>[2x]MGLASLADFPIGVAVAASGGNADIFTSSARQNIVRAEFNQITAENIMKMSYMYSGSNFSFTNSDRLVSWAAQN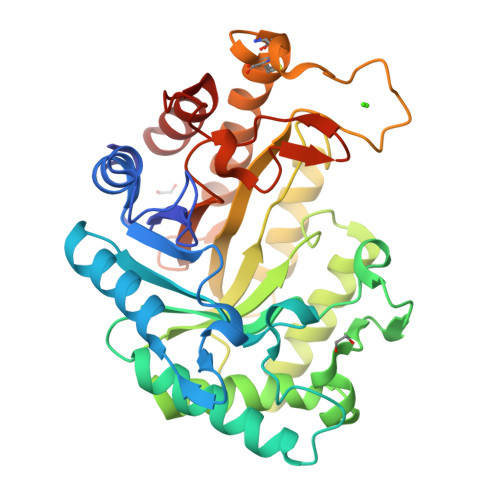GQTVHGHALVWHPSYQLPNWASDSNANFRQDFARHIDTVAAHFAGQVKSWDVVNEALFDSADDPDGRGSANGYRQSVFYRQFGGPEYIDEAFRRARAADPTAELYYNDFNTEENGAKTTALVNLVQRLLNNGVPIDGVGFQMHVMNDYPSIANIRQAMQKIVALSPTLKIKITELDVRLNNPYDGNSSNNYTNRNDCAVSCAGLDRQKARYKEIVQAYLEVVPPGRRGGITVWGIADPDSWLYTHQNLPDWPLLFNDNLQPKPAYQGVVEALSGR>MRGSHHHHHHGSMSNKI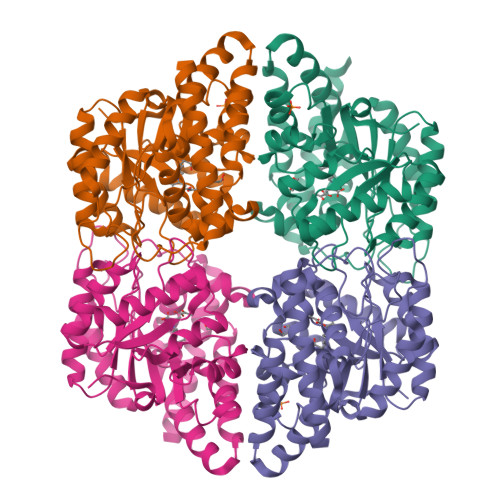MKTSRLTAEDINGAWTIMPTPSTPDASDWRSTATVDLEETARIVEELIAAGVNGILSMGTFGECATLTWDEKRDYVSTIVETIRGRVPYFCGTTALNTREVIRQTRELIDIGANGTMLGVPMWVKMDLPTAVQFYRDVADAVPEAAIAIYANPEAFKFDFPRPFWAEMSKIPQVVTAKYLGIGMLDLDLRLAPNIRFLPHEDDYYAAARINPERITAFWSSGAMCGPATAIMLRDEVVRAKSTGDWAKAKAISDDMRAADSTLFPRGDFSEFSKYNIGLEKARMDAAGWLKAGPCRPPYNLVPEDYLAGAQKSGKAWAALHAKYSNELK[8x]>[2x]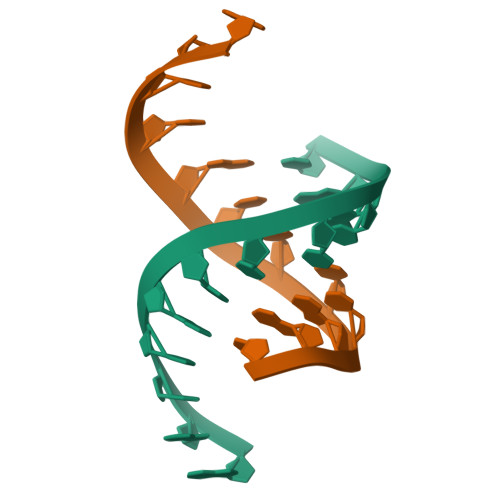GAUCACUUCGGU> 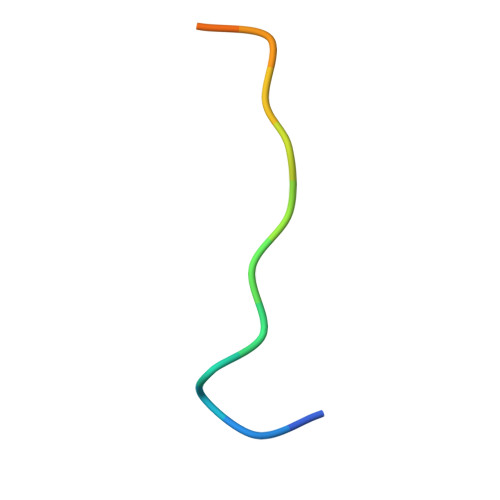FNDNYSSTSTVYATS> GMELPVVVQQALGDNAPGVSFRSVSQIDTGHLLRMVLLSDDQGNLQAICRRNDMLDLEALNKRLGRDLRMMQRREQVRVRQKAGLQELPALPSLTGWPTVVDRRVDELEAVALELGEQDLGLMMPAEDFRQLTAKAARHDFAVDTANISVNLDNHAADRDQLHSAIKRFTGLRIQQRLEDTLELPPLPETAQRIIHLRVNPNAVMGDLVDVVESDPSLAAQVVSWASSSFYAAAGRVHSVHDAVSRVLGFDLVMNLAMGLALGRALKHPQDHPDGYVDYWQQAIWQAQSAGILASMMPRGQRPLFGLAYLAGLLHNFGHLVLAQVFPPHFKLVCRSLEVSPHIDSSVIEHYLLGITREQIAAQLMENWGMPDEVTLAIRYQKNPAYDGPHNVYARLLWLGRQLLTERGVALGAGESATQAVYDELGLDRELVQEQFDELV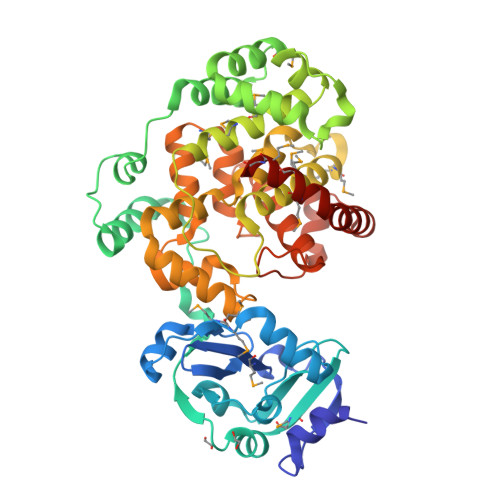RRKDSIMAMAGMMSQGG> SNAMFAPQGLAQFIKVNVTLENGEPVFIYTDANGQVCQGD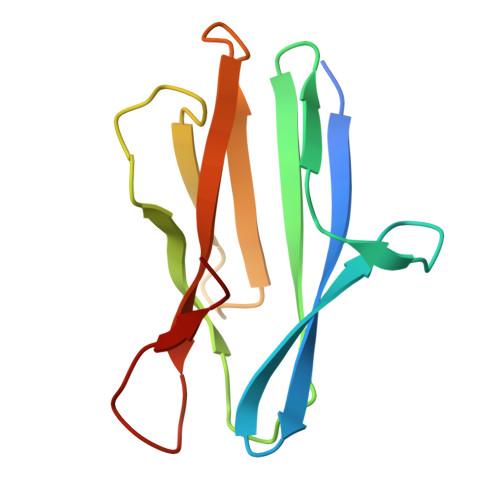ITVTQAGTITYLLNDQTLKGLKFVGVGFVTPFDGIIDAVTISSDGMLVQLVDLDKTPGTTKFQFVLSNTANTLLVLSAD Sapovirus (SaV) belongs to the *Caliciviridae* family and is well known to cause acute gastroenteritis in humans as well as animals. The major capsid protein VP1 is solely responsible for most capsid-related functions, such as assembly, host interactions, and immunogenicity. The calicivirus virions have a mostly conserved capsid shell, which is composed of 180 copies of VP1 arranged in a T=3 icosahedral symmetry. Each VP1 capsid monomer contains two principal domains, shell (S) and protrusion (P) domains, with an N-terminal arm located inside the capsid shell.

Here, we determined the capsid structure of a HuSaV virus-like particle (HuSaV-VLP) at 2.9 Å resolution by single particle cryo-electron microscopy (cryo-EM), and successfully built an atomic model of the capsid. The cryo-EM map clearly shows a T=3 icosahedral symmetry with 90 protrusions, composed of 180 copies of the VP1 protein in total, distributed along the icosahedral 2-fold axes (C/C dimers) and quasi 2-fold axes (A/B dimers) on the surface ([Fig fig1] and S2A). The cryo-EM map allowed atomic modeling of residues 38–554 for subunit A, residues 21–554 for subunit B, and residues 21–554 for subunit C, except for one disordered loop (residues 380–384) for all subunits ([Fig fig2]). The icosahedrally independent A/B and C/C dimers show slightly different conformations, mainly between S-domains in each dimer, which are the bent and flat conformations, respectively, as in other T=3 viruses. In addition, N-terminal regions of residues 21–37 in the B- and C-subunits extend underneath the capsid shell and interact with the neighboring subunits around icosahedral 3-fold axes ([Fig fig3]), although the N-terminal region is disordered in the A-subunit, and no N-terminal network is observed around icosahedral 5-fold axes. Therefore, the N-terminal network around the icosahedral 3-fold axes likely stabilized the hexameric units in the capsid. The P domain is further divided into two subdomains, P1 (233–281 and residues 444–554) and P2 (residues 282–443) subdomains. Unexpectedly, in addition to the residues in the P2 subdomain, the residues in the P1 subdomain are involved in the interaction between the P domains ([Fig fig6]). The βB’-α4 loop (residues 465–469) in the P1 subdomain and the βC”-βD” loop in the P2 subdomain are mainly involved in the interaction between the P domains. In particular, residues 294–306 in βA”-βB”, 337–347 in βB”-βC”, 375–388 in βD”-βE” (including a disordered region, 380–384), and 403–417 in βE”-βF” show significant sequence variabilities between the HuSaVs, which are designated as hypervariable region 1 (HVR1), HVR2, HVR3, and HVR4, respectively ([Fig fig4]).

>MEGNGSQLGSRQHQESQAAVDPPGATGPTTSHVVVSNPEQPNGPAQRLEMAVATGAIQSNVPEAIRNCFAVYRTFAWNDRMPAGTFLGSVSLHPNINPYTSHLSGMWAGWGGSFESRVSISGSGVFAGRVVASVIPPGVDPSSIRDPGVLPHAFVDARITEPVSFMIPDVRNTDYHRMDGNEPTCSLGLWVYQPLINPFSTSAVSTCWVSIETKPGGDFDFCLLKPPGQRMENGVSPEGLLPRRLGYARGNRVGGLVVGLVLVADHHQVNRHFNANSITYGWSTAPVNPMAAEIVVKHDYTNNRNAWLSIGAKNKGPLFPGLPNHFPDSCASTLVGAMDTGRHMPATGVCGPAIGFQDNGDVFENETPAVMFATFNPLTGGDNTNPIALYDSINPASLAVMCTKSNSNFDSSGFANDKNVVVQMSWEMYTNSQQIQGRVTPMQGTNFVFTSSGANTLALWEERLLSYDGHQAILYSSQMERTSEYFQNDNVNIPPGSMAVFNVETNSASFQIGIREDGYMVTGGTIGTHVVLDPETRFQYVGLLPLTAALAGPNGNSGRARRVFQ[3x]> MAHMTTSYAKIEITGTLTVLTGLQIGAGDGFSAIGAVDKPVVRDPLSRLPMIPGTSLKGKVRTLLSRQYGADTETFYRKPNEDHAHIRRLFGDTEEYMTGRLVFRDTKLTNKDDLEARGAKTLTEVKFENAINRVTAKANLRQMERVIPGSEFAFSLVYEVSFGTPGEEQKASLPSSDEIIEDFNAIARGLKLLELDYLGGS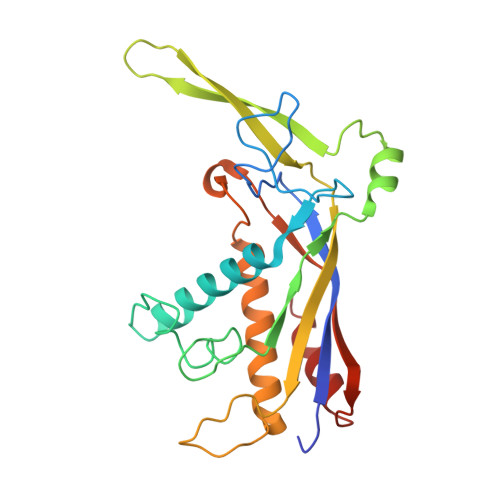GTRGYGQVKFSNLKARAAVGALDGSLLEKLNHELAAV> MSNQDALFHSVKDDIHFDTLLEQAHQVIEKQAEKLWSDTAEHDPGITFLQGISYGVSDLAYRHTLPLKDLLTPAPDEQQQEGIFPAEFGPHNTLTCGPVTADDYRKALLDLHSSDSLDGTQQDEGDFLFRSVQLVREPEKQRYTYWYDATKREYSFVNSEGAKEFTLRGNYWLYLEPTRWTQGNIAAATRQLTEFLTKNRNIGESVSNIIWLQPVDLPLLLDVELDDDVGAQDVPGIFAAVYSTAEQYLMPGAQRYRTEVLQNAGMSNDQIFEGPLLEHGWIPELPAARDYTQRLTLNLSRLVNSLLEIEGIKHVNRLRLDDSFDKTAIEPVKGDTWSWSIKEGYYPRLWGEDPLNQLAQQNGPLRVIAKGGISVSVSKEQIQASLPSQSLIQNEPVILAYGQHRDVGSYYPVSDTLPPCYGLQHSLSESEHLLPLHQFMLPFEQLLACGCQQIAMLPRLLAFQREGYEVWGDQWPFKSGSVNDDAHQDYAPALKDLLGQIALDSDHELDIINYLLGYFGTQRAPRTFTTQLDDFRAVQQGYLAQQPTLTYHRSNIRIDQVSSLQKRIAARMGLGGELFKPQPDLSQLPFYLIEHRALLPVKPNSQFDKEQKPASVTEEGGSQTGQHYVVIEQKGIDGKLTQGQVINLILYEGEQGETQFTIRGQMVFKTEGDKFWLDVNNSAQLEYNLARVMTAAKASKLF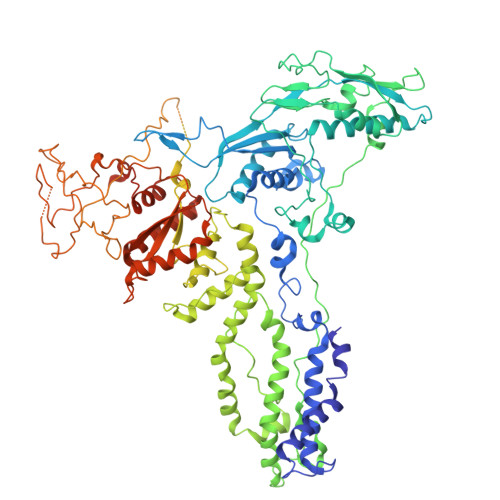WQNSPVWMEDMGYRLAYASDQSSLPVNQRRLTRTVQTPFPPMVVVGSEITLLKQVGIVNLKKAESEKLYAKVVSFDRIEGTLIIERLGNSTLAFPTSEEAWRYSWYFSGEKYERTDRFSFVISVVVNSDLIKLPGVDPYKLEEWVKETILTEFPAHISMIIHWMDREAFLNFANTYQRWQNNGTPLGDAAYSILESLTLGKLPSALKGVGTMRIATSSQREEVVGSNGDQWNTDGITQNELFYVPKES>[2x]MRGSHHHHHHGSTVDKVKLVIDSDGVSDDVRAISLALQHPKAEILAFTAVHGCVTVDQACANIKRTIRANDRSNIPVYKGAAKSILSLPKDDTVSDFFGIDGIGDKPEEFP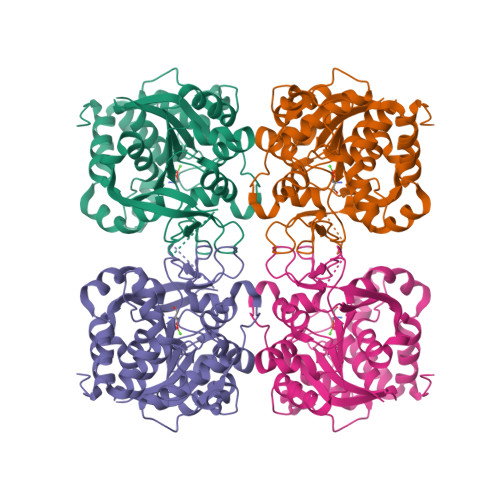KVERSDFEGEGKHASLALIDILRENRDATLVTIGPLTNVAIALQLCEEFSTYPSRLVIMGGNYYAVGNVDGGSSAEYNFHGDPEAASIVLRRMKCPITIVPWEAFYFESKTHDASVDFSAHLKYGTPLANYLSLATSIGRVKCEANGRQYSYCDEIAVATAIDEDKIAKKSQYLYVDVELNGTKTRGQVVVDWTEQLWSNEEAPNQHTHRRVKFVTSYDVHTVDKWLHAATSGSGKFD Phage portal proteins are key viral components located in a single pentameric vertex of the capsid and they act as initiators of capsid assembly. They are also critical components of the DNA-packaging complex and are involved in tail assembly. Here we report a number of crystal and high-resolution cryo-electron microscopy (cryo-EM) structures of the T7 bacteriophage portal (gp8). The structures show two conformations—open and closed—of the portal and suggest a possible mechanism of the channel valve that regulates DNA passage.

The gp8 monomeric structure was then used for phasing the gp8-12mer 3.6 Å resolution crystallographic data (gp8closed, see Methods section), which yielded an atomic model of the dodecameric portal. The overall shape of the T7 portal protein shows a ring-like assembly formed by 12 subunits and with an axial central channel. The external diameter of the particle is 170 Å, whereas its height is 110 Å. The diameter of the channel (measured between opposite Cα atoms) is 23 Å at its narrowest section, which would hinder the passage of a B-DNA molecule. Regarding the shape of the portal central channel, there are two cavities, “upper” and “bottom”, with a conical and an inverted conical shape, respectively, separated by the protrusion of α10 toward the center of the channel. The electrostatic potential of the protein is markedly negative, both on the external and inner surfaces, except for the exterior of the clip and the tunnel loop, due to R368. The tunnel loop, a singular feature also found in other portal particles, is between α9 and α10, and only partially observable in the gp8 dodecameric structure due to its intrinsic flexibility. Therefore, two clearly different conformations in the T7 connector were defined: one closed (gp8closed) and the other open (gp8open). Although the first structure described in this work (gp8closed) would impede the DNA passage through it, the second structure (gp8open) would allow it. The closure of the T7 portal protein, as observed here, does not allow the passage of the genome and therefore the portal valve is likely to be in the open conformation during DNA packaging.

>[12x]RTGLAEDGAKSVYERLKNDRAPYETRAQNCAQYTIPSLFPKDSDNASTDYQTPWQAVGARGLNNLASKLMLALFPMQTWMRLTISEYEAKQLLSDPDGLAKVDEGLSMVERIIMNYIESNSYRVTLFEALKQLVVAGNVLLYLPEPEGSNYNPMKLYRLSSYVVQRDAFGNVLQMVTRDQIAFGALPEDIRKAVEGQGGEKKADETIDVYTHIYLDEDSGEYLRYEEVEGMEVQGSDGTYPKEACPYIPIRMVRLDGESYGRSYIEEYLGDLRSLENLQEAIVKMSMISSKVIGLVNPAGITQPRRLTKAQTGDFVTGRPEDISFLQLEKQADFTVAKAVSDAIEARLSFAFMLNSAVQRTGERVTAEEIRYVASELEDTLGGVYSILSQELQLPLVRVLLKQLQATQQIPELPKEAVEPTISTGLEAIGRGQDLDKLERCVTAWAALAPMRDDPDINLAMIKLRIANAIGIDTSGILLTEEQKQQKMAQ> MKHLISMKDIGKEEILEILDEARKMEELLNTKRPLKLLEGKILATVFYEPSTRTRLSFETAMKRLGGEVITMTDLKSSSVAKGESLIDTIRVISGYADIIVLRHPSEGAARLASEYSQVPIINAGDGSNQHPTQTLLDLYTIMREIGRIDGIKIAFVGDLKYGRTVHSLVYALSLFENVEMYFVSPKELRLPKDIIEDLKAKNIKFYEKESLDDLDDDIDVLYVTRIQKERFPDPNEYEKVKGSYKIKREYVEGKKFIIMHPLPRVDEIDYDVDDLPQAKYFKQSFYGIPVRMAIL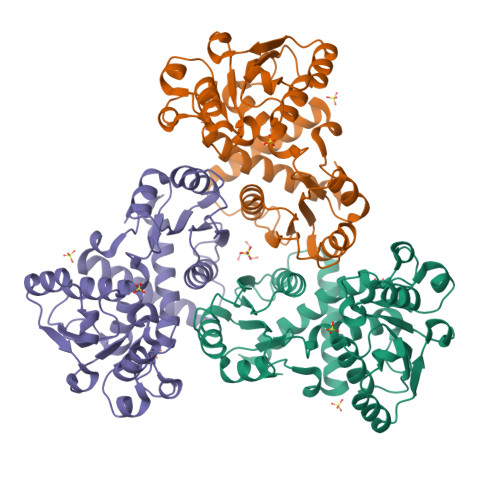KKLIEDNEGE> XMEVCLPNGHQIVDLINNAFEGRVSIYSAQEGWDKTISAQPDMMVCGGAVVCMHCLGVVGSLQRKLKHLPHHRCNQQIRHQDYVDVQFADRVTAHWKRGMLSFVCQMHAMMNDVSPEDLDRVRTEGGSLVELNWLQVDPNSMFRSIHSSWTDPL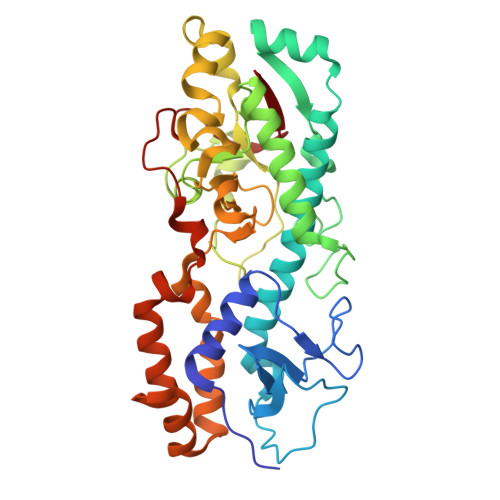QVVDDLDTKLDQYWTALNLMIDSSDLVPNFMMRDPSHAFNGVRLEGDARQTQFSRTFDSRSSLEWGVMVYDYSELEHDPSKGRAYRKELVTPARDFGHFGLSHYSRATTPILGKMPAVFSGMLTGNCKMYPFIKGTAKLKTVRKLVDSVNHAWGVEKIRYALGPGGMTGWYNRTMQQAPIVLTPAALTMFSDTTKFGDLDYPVMIGDPMILG>[4x]ISSQAVTSVPYKWDNVVIGGGGGFMPGIVFNETEKDLIYARADIGGAYRWDPSTETWIPLLDHFQMDEYSYYGVESIATDPVDPNRVYIVAGMYTNDWLPNMGAILRSTDRGETWEKTILPFKMGGNMPGRSMGERLAIDPNDNRILYLGTRCGNGLWRSTDYGVTWSKVESFPNPGTYIYDPNFDYTKDIIGVVWVVFDKSSSTPGNPTKTIYVGVADKNESIYRSTDGGVTWKAVPGQPKGLLPHHGVLASNGMLYITYGDTCGPYDGNGKGQVWKFNTRTGEWIDITPIPYSSSDNRFCFAGLAVDRQNPDIIMVTSMNAWWPDEYIFRSTDGGATWKNIWEWGMYPERILHYEIDISAAPWLDWGTEKQLPEINPKLGWMIGDIEIDPFNSDRMMYVTGATIYGCDNLTDWDRGGKVKIEVKATGIEECAVLDLVSPPEGAPLVSAVGDLVGFVHDDLKVGPKKMHVPSYSSGTGIDYAELVPNFMALVA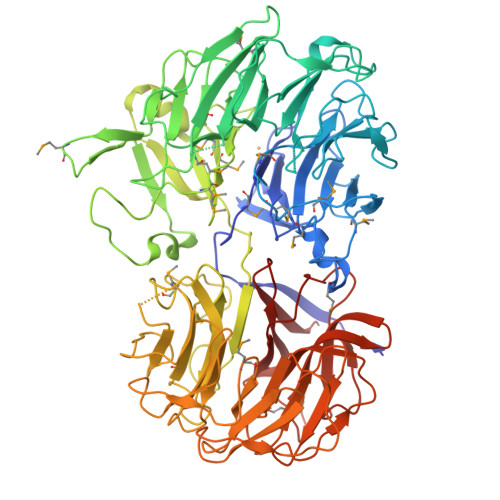KADLYDVKKISFSYDGGRNWFQPPNEAPNSVGGGSVAVAADAKSVIWTPENASPAVTTDNGNSWKVCTNLGMGAVVASDRVNGKKFYAFYNGKFYISTDGGLTFTDTKAPQLPKSVNKIKAVPGKEGHVWLAAREGGLWRSTDGGYTFEKLSNVDTAHVVGFGKAAPGQDYMAIYITGKIDNVLGFFRSDDAGKTWVRINDDEHGYGAVDTAITGDPRVYGRVYIATNGRGIVYGEPASDEPV>MKTSEQRVNIATLLTENKKKIVDKASQDLWRRHPDLIAPGGIAFSQRDRALCLRDYGWFLHLITFCLLAGDKGPIESIGLISIREMYNSLGVPVPAMMESIRCLKEASLSLLDEEDANETAPYFDYIIKAMSEFHHHHHH[6x]

Our previous efforts to develop a far-red FP with improved performance relative to other FPs yielded the small Ultra-Red FP (smURFP), which we created from the α-allophycocyanin phycobiliprotein through 12 rounds of directed evolution. Unlike α-allophycocyanin phycobiliprotein which requires a lyase to attach the chromophore, smURFP formed a covalent bond with BV via a cysteine residue without needing a lyase. Furthermore, smURFP is small (16 kD) relative to the GFP (27 kD), and yet its molecular brightness is equivalent to the enhanced GFP (eGFP) with a fluorescence quantum yield (QY) of 18% and a large extinction coefficient (EC) of 180,000 M−1 cm−1 at 642 nm1,11,12. smURFP was successfully incorporated into genetically encoded far-red and near-IR ubiquitination-based cell cycle indicator (FUCCI)11 and Förster resonance energy transfer (FRET) kinase sensor. The structure reveals that smURFP is a homodimer, and polar, π-π, and hydrophobic interactions mediate dimer formation.

On the other hand, apo-smURFP crystallized from a solution of smURFP with 20% BV attached, enabling us to determine the structure at 2.8 Å resolution. We observed that the asymmetric unit contains a hexamer with three smURFP homodimers. Each smURFP monomer comprises six alpha helixes (h1-h6) connected by loops. Two monomers form a dimer through hydrogen bonds and polar, π-π, and hydrophobic interactions at the dimeric interface. The interface is also stabilized by two salt bridges between h2 and h3 (K18, K19 to D55 and D23 to R54) and a π-π interaction between F65 of h3 from each monomer. Hydrophobic interactions also contribute to the interface, most notably L68 of h3 and I78 of h4 of the counterpart. In our structure, we observed that C52 is located at the edge of h3 within a pocket that binds and subsequently covalently attaches BV. Importantly, the smURFP chromophore pocket is formed by amino acids from both protomers, which agreed with our previous directed evolution studies that indicated that the dimer was required for BV incorporation. Whereas allophycocyanin hexamer is composed of three heterodimers of αβ subunits that partially overlap side-by-side to form a hollow disc, the three homodimers of smURFP form a smaller pinwheel-like structure. The comparison of the chromophore pockets revealed that the pocket in the smURFP Y56F mutant was larger at 663 Å3 with disordered loops compared to smURFP, which forms a smaller pocket (576 Å3) with a compact and rigid secondary structure.> 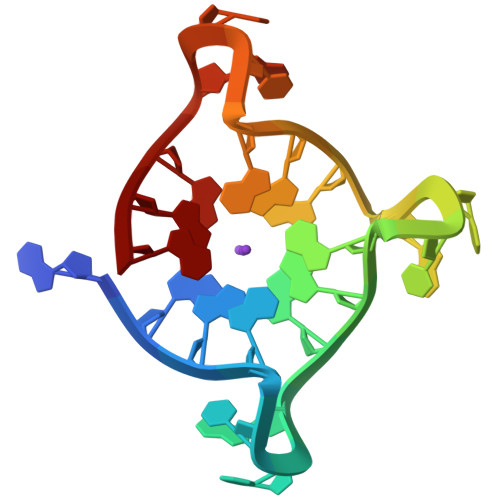AGGGTTAGGGTXAGGGTTAGGG>MLKVSKSPSLVRLKTRGESVCPISKTVDSFEVSVEYIPRGAVLAIEEFKKMVDSYRGREILHEELAVDLLEKVKAAVNPPYVKVTVKSYYIGVE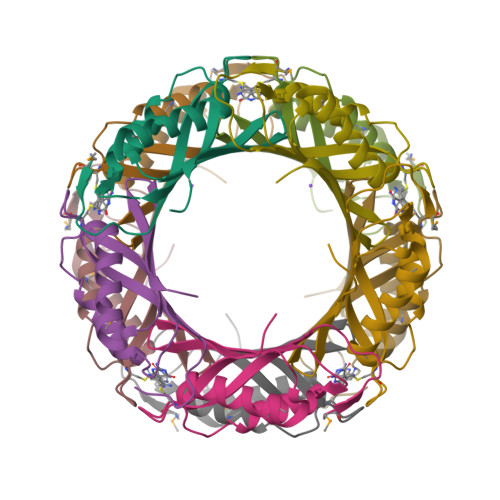VEVVAESGGVPPVYI[15x]>HHHHHHMSSSEVDKVFTEEQEALVVKSWAVMKKNSAELGLKFFLKIFEIAPSAKNLFSYLKDSPIPLEQNPKLKPHAMTVFVMTCESAVQLRKAGKVTVRESNLKRLGAIHFKNGVVNEHFEVTRFALLETI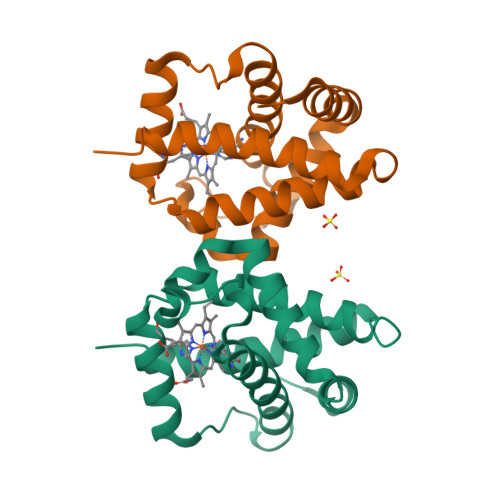KEAVPEMWSPEMKNAWGEAYDQLVAAIKSEMKPSST[2x]> MSRQASRLDAKKVNSEFLTLTYGALVTQMLRDFENAEDVNKQLERIGYNMGMRLIEDFLARTSAPRCLEMRETADRIQQAFRIYLNIQPTISNWSPASDEFSLVFDSNPLTEFVELPPDLTNLRYSAILSGCIRGALEMVQLEVQCW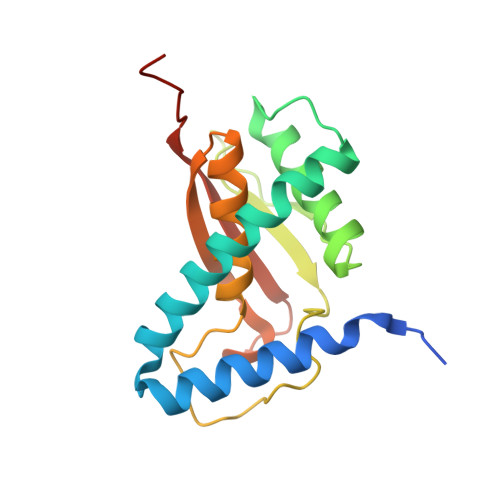FVQDQLKGDNVTELRVKFVRRLEEVIPAGED> GPGSGQLLFANFNQDNTSLAVGSKSGYKFFSLSSVDKLEQIYECTDTEDVCIVERLFSSSLVAIVSLKAPRKLKVCHFKKGTEICNYSY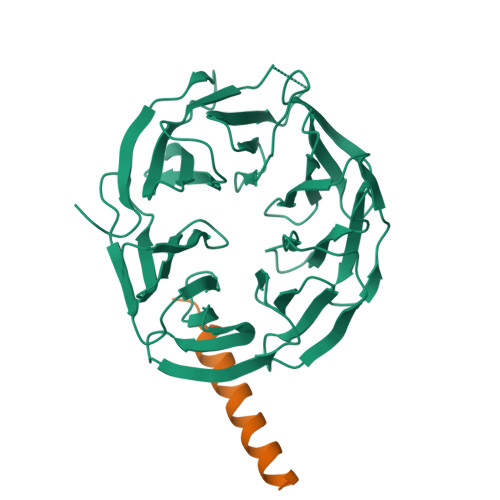SNTILAVKLNRQRLIVCLEESLYIHNIRDMKVLHTIRETPPNPAGLCALSINNDNCYLAYPGSATIGEVQVFDTINLRAANMIPAHDSPLAALAFDASGTKLATASEKGTVIRVFSIPEGQKLFEFRRGVKRCVSICSLAFSMDGMFLSASSNTETVHIFKLETVKEKPPEEPTTWTGYFGKVLMASTSYLPSQVTEMFNQGRAFATVRLPFCGHKNICSLATIQKIPRLLVGAADGYLYMYNLDPQEGGECALMKQHRLDGSLV;> GPGSAENEKDSRRRQARLQKELAEAAKEPLPVEQ4-[(3-carboxy-2-oxidanyl-naphthalen-1-yl)methyl]-3-oxidanyl-naphthalene-2-carboxylic acid | C23 H16 O6 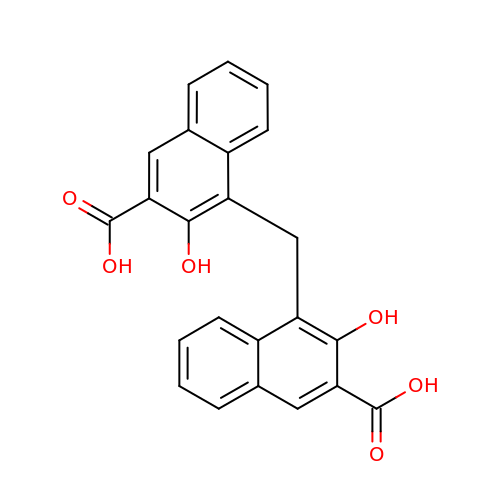| WLJNZVDCPSBLRP-UHFFFAOYSA-N> MGQSEKQEEPDYPINKFMNTTDEIWVFRTTQENVQKCKKDKNKYMTTSATFFTRSHEEQDQIHEQELVGKFANFYDKPDGVYDRIDITGDKTGVYEEALAYASKENTCGVVGVWAFDGETTVVWRELRVRNRPNDATKVDEMCKKKFDDYVQVVNKSWTSPYNEKCK

In this study, we identify a family of complement inhibitors from the hard tick Rhipicephalus pulchellus, hereafter termed CirpA (Complement inhibitor from R. pulchellus of the alternative pathway). Functional and structural characterisation reveals that members of the CirpA family directly bind to properdin, inhibiting its ability to promote complement activation, and leading to potent inhibition of the complement response in a species specific manner. Whilst many molecules act to control inappropriate activation, Properdin is the only known positive regulator of the human complement system. All CirpA structures share a lipocalin fold with a short N-terminal α-helix followed by an eight-stranded beta-barrel and a longer C-terminal α-helix.

Using this strategy, we were able to purify CirpA1, A3, A4, and A5 and determine their structure using X-ray crystallography to a resolution of 2.0, 2.1, 1.8, and 1.9 Å respectively. Overall, the structures appear very similar, with the biggest conformational differences in the tilt angle of the C-terminal helix H2 as well as variations in loops between beta strands 4 and 5 (L4-5) and between strands 7 and 8 (L7-8). We identified three regions with high conformational variability between homologs. All these regions are part of the observed binding interface between CirpA1 and properdin, and hence the conformational differences might render other homologs incompatible with binding human properdin. Another CirpA1 residue undergoing a conformational rearrangement upon properdin binding is Y122 which forms a hydrophobic pocket around properdin P377 together with CirpA1 residues F122, Y131, and F150. This pocket is incomplete in all three CirpA1 homolog structures. However, it is likely that the homologues have evolved to target properdin from other species, especially given the identification of multiple CirpA homologues in a single tick species.> CGGAGGAACUACUGUCUUCACGCC;> GC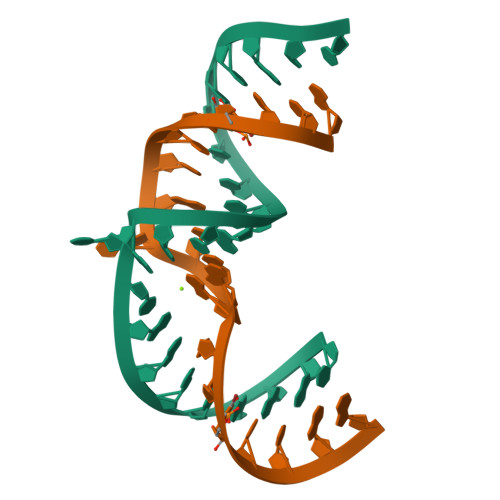GUGUCGUGCAGCCUCCGG> MKVEELIIDGFKSYATRTVITDWDPQFNAITGLNGSGKSNILDAICFVLGIASMSTVRASSLQDLIYKRGQAGVTKASVTIVFDNTDKSNSPIGFTNSPQISVTRQVVLGGTSKYLINGHRAPQQSVLQLFQSVQLNINNPNFLIMQGKITKVLNMKPSEILSLIEEAAGTKMFEDRREKAERTMSKKETKLQENRTLLTEEIEPKLEKLRNEKRMFLEFQSTQTDLEKTERIVVSYEYYNIKHKHTSIRETLENGETRMKMLNEFVKKTSEEIDSLNEDVEEIKLQKEKELHKEGTISKLENKENGLLNEISRLKTSLSIKVENLNDTTEKSKALESEIASSSAKLIEKKSAYANTEKDYKMVQEQLSKQRDLYKRKEELVSTLTTGISSTGAADGGYNAQLAKAKTELNEVSLAIKKSSMKMELLKKELLTIEPKLKEATKDNELNVKHVKQCQETCDKLRARLVEYGFDPSRIKDLKQREDKLKSHYYQTCKNSEYLKRRVTNLEFNYTKPYPNFEASFVHGVVGQLFQIDNDNIRYATALQTCAGGRLFNVVVQDSQTATQLLERGRLRKRVTIIPLDKIYTRPISSQVLDLAKKIAPGKVELAINLIRFDESITKAMEFIFGNSLICEDPETAKKITFHPKIRARSITLQGDVYDPEGTLSGGSRNTSESLLVDIQKYNQIQKQIETIQADLNHVTEELQTQYATSQKTKTIQSDLNLSLHKLDLAKRNLDANPSSQIIARNEEILRDIGECENEIKTKQMSLKKCQEEVSTIEKDMKEYDSDKGSKLNELKKELKLLAKELEEQESESERKYDLFQNLELETEQLSSELDSNKTLLHNHLKSIESLKLENSDLEGKIRGVEDDLVTVQTELNEEKKRLMDIDDELNELETLIKKKQDEKKSSELELQKLVHDLNKYKSNTNNMEKIIEDLRQKHEFLEDFDLVRNIVKQNEGIDLDTYRERSKQLNEKFQELRKKVNPNIMNMIENVEKKEAALKTMIKTIEKDKMKIQETISKLNEYKRETLVKTWEKVTLDFGNIFADLLPNSFAKLVPCEGKDVTQGLEVKVKLGNIWKESLIELSGGQRSLIALSLIMALLQFRPAPMYILDEVDAALDLSHTQNIGHLIKTRFKGSQFIVVSLKEGMFANANRVFRTRFQDGTSVVSIMXXXXXXXX;> MSDSPLSKRQKRKSAQEPELSLDQGDAEEDSQVENRVNLSENTPEPDLPALEASYSKSYTPRKLVLSSGENRYAFSQPTNSTTTSLHVPNLQPPKTSSRGRDHKSYSQSPPRSPGRSPTRRLELLQLSPVKNSRVELQKIYDRHQSSSKQQSRLFINELVLENFKSYAGKQVVGPFHTSFSAVVGPNGSGKSNVIDSMLFVFGFRANKMRQDRLSDLIHKSEAFPSLQSCSVAVHFQYVIDESSGTSRIDEEKPGLIITRKAFKNNSSKYYINEKESSYTEVTKLLKNEGIDLDHKRFLILQGEVENIAQMKPKAEKESDDGLLEYLEDIIGTANYKPLIEERMGQIENLNEVCLEKENRFEIVDREKNSLESGKETALEFLEKEKQLTLLRSKLFQFKLLQSNSKLASTLEKISSSNKDLEDEKMKFQESLKKVDEIKAQRKEIKDRISSCSSKEKTLVLERRELEGTRVSLEERTKNLVSKMEKAEKTLKSTKHSISEAENMLEELRGQQTEHETEIKDLTQLLEKERSILDDIKLSLKDKTKNISAEIIRHEKELEPWDLQLQEKESQIQLAESELSLLEETQAKLKKNVETLEEKILAKKTHKQELQDLILDLKKKLNSLKDERSQGEKNFTSAHLKLKEMQKVLNAHRQRAMEARSSLSKAQNKSKVLTALSRLQKSGRINGFHGRLGDLGVIDDSFDVAISTACPRLDDVVVDTVECAQHCIDYLRKNKLGYARFILLDRLRQFNLQPISTPENVPRLFDLVKPKNPKFSNAFYSVLRDTLVAQNLKQANNVAYGKKRFRVVTVDGKLIDISGTMSGGGNHVAKGLMKLGTNQSDKVDDYTPEEVDKIERELSERENNFRVASDTVHEMEEELKKLRDHEPDLESQISKAEMEADSLASELTLAEQQVKEAEMAYVKAVSDKAQLNVVMKNLERLRGEYNDLQSETKTKKEKIKGLQDEIMKIGGIKLQMQNSKVESVCQKLDILVAKLKKVKSASKKSGGDVVKFQKLLQNSERDVELSSDELKVIEEQLKHTKLALAENDTNMNETLNLKVELKEQSEQLKEQMEDMEESINEFKSIEIEMKNKLEKLNSLLTYIKSEITQQEKGLNELSIRDVTHTLGMLDDNKMDSVKEDVKNNQELDQEYRSCETQDESEIKDAETSCDNYHPMNIDETSDEVSRGIPRLSEDELRELDVELIESKINELSYYVEETNVDIGVLEEYARRLAEFKRRKLDLNNAVQKRDEVKEQLGILKKKRFDEFMAGFNIISMTLKEMYQMITMGGNAELELVDSLDPFSEGVTFSVMPPKKSWRNITNLSGGEKTLSSLALVFALHKYKPTPLYVMDEIDAALDFRNVSIVANYIKERTKNAQFIVISLRNNMFELAQQLVGVYKRDNRTKSTTIKNIDILNRT;> MTTQLRYENNDDDERVEYNLFTNRSTMMANFEEWIKMATDNKINSRNSWNFALIDYFYDLDVLKDGENNINFQKASATLDGCIKIYSSRVDSVTTETGKLLSGLAQRKTNGASNGDDSNGGNGEGLGGDSDEANIEIDPLTGMPISNDPDVNNTRRRVYNRVLETTLVEFETIKMKELDQELIIDPLFKKALVDFDEGGAKSLLLNTLNIDNTARVIFDASIKDTQNVGQGKLQRKEEELIERDSLVDDENEPSQSLISTRNDSTVNDSVISAPSMEDEILSLGMDFIKFDQIAVCEISGSIEQLRNVVEDINQAKDFIENVNNRFDNFLTEEELQAAVPDNAEDDSDGFDMGMQQELCYPDENHDNTSHDEQDDDNVNSTTGSIFEKDLMAYFDENLNRNWRGREHWKVRNFKKANLVNKESDLLEETRTTIGDTTDKNTTDDKSMDTKKKHKQKKVLEIDFFKTDDSFEDKVFASKGRTKIDMPIKNRKNDTHYLLPDDFHFSTDRITRLFIKPGQKMSLFSHRKHTRGDVSSGLFEKSTVSANHSNNDIPTIADEHFWADNYERKEQEEKEKEQSKEVGDVVGGALDNPFEDDMDGVDFNQAFEGTDDNEEASVKLDLQDDEDHKFPIRENKVTYSRVSKKVDVRRLKKNVWRSINNLIQEHDSRKNREQSSNDSETHTEDESTKELKFSDIIQGISKMYSDDTLKDISTSFCFICLLHLANEHGLQITHTENYNDLIVNYEDLATTQAASXXXXXXXXXXXXXXXXXXX;> MSGFSLSEYLTKFQTTDRESYPRLQDPSRELNVIIDQLAVSPEQIDASPDSLEALIDLCHDFPHLTPKLQTQLSYLISSSLSNLSKDIKANLSSNVNFTEIGGLIPQWKRHLEEYGYLIQVLLTFLQDELHKVSSQSTNLNRSAKNSKNDSANVELFKRDCNQMENLLESITKLLEINLSKIFQTTPEKDLFIGLFTRPLFVLLEIEPVTKVSSLKMFIQRILAMCVKNHGQSSSIQSSLMTNLTYFLHLSVFNAELLKLLNDEYNYPQLTEDILKEISTRVFNAKDTTGPKAISNFLIKLSELSPGIMLRQMNLVITLLNNSSITLRCSVVEACGNIVAELAQDPQTMEHYKQQIAVLIELLEERFQDSNPYVRTKAIQGCSKICDLSSKFNKSKAKFTSLAVRSLQDRSSLVRRNSVKLLSKLLLKHPFKAIHGSQLRLSEWEEYLKGSESQLNSTLKKVESQETLNDTIERSLIEEEVEQDEGQCRTELEGSFNKSAELSRIENEVENINATNTSVLMKLKLMIVYYKDAISFIKEIHKSIELISNLLFSKNRNEVLESMDFLVLADAFDIELSEFGIKKMLHLVWMKGTNDEGTSISVHLIECYKQLFLTAPDSCNMQEKAAHIAKNLINLSIGASIADLASLEQLLGMMYEQKLIDQHVINILWAIYNSASKASMQKEQNVNNRDSEKGFSKEQIHGSIIILGMLSLADNEIALKGLESLLNIGLGAVGLKDLTLCRYSCLALERMVPKRSTIITKAINQELEDVAVKKLYAIIINYTKDNEYYPMCEQALSALFTIS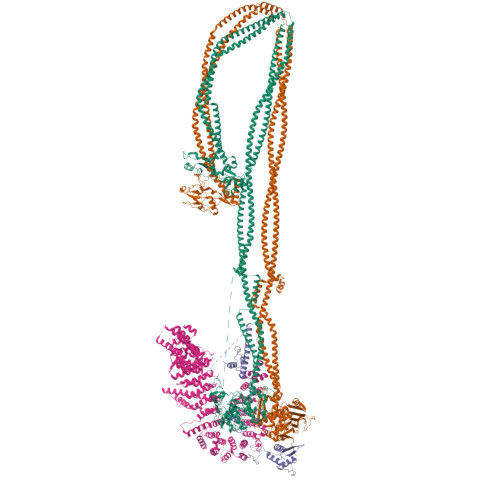SKPDILATDLIREKTMMTFGKPEEEDSILSLEQSSRVVSLSQLLFIVGQVAIKTLVYLEKCEAEFKKRKIEAETRNGKVKNQGADVTNTTQDNGGDKELEMIGGTNEDDFTDAIQFVKENELLFGEKSILGKFCPIVEEIVSNSSRFSDPMLQRTATLCLEKLMCLSSKYCEKSLPLLITVMEKSPDPTIRSNAVLGLGDMAVCFNNLVDENTDYLYRRLHDENLMVQRTCLMTVTFLILAGQVKVKGQLGEMAKCLDNPDQGISDMCRLFFTELASKDNAIYNGFIDIFSNLSSDDLLGKESFKKIIKFLLTFIDKERHQKQLNEKLVGRLRKCETQKQWDDIAFVLNNLPYKNEDVTALLEQGFKVVSAKEXXXXXXXXX5-chloro-2-methoxy-N-([1,2,4]triazolo[1,5-a]pyridin-8-yl)benzene-1-sulfonamide | C13 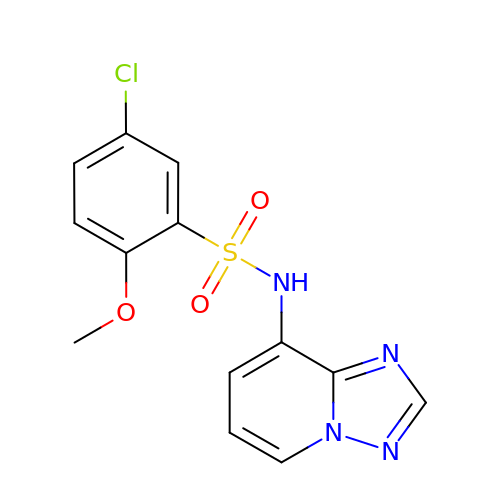H11 Cl N4 O3 S | VLSIKQJXWTXQPQ-UHFFFAOYSA-N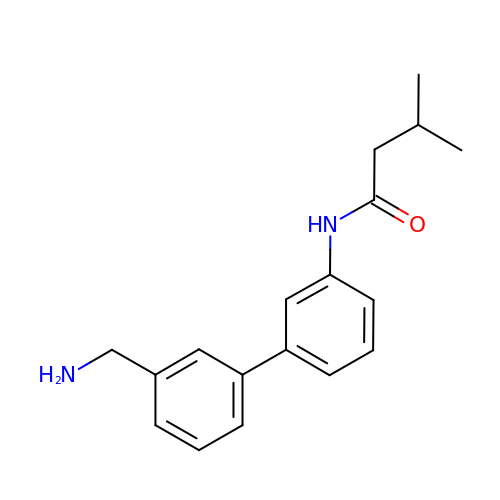~{N}-[3-[3-(aminomethyl)phenyl]phenyl]-3-methyl-butanamide | C18 H22 N2 O | ZTMBFIOZACRTLO-UHFFFAOYSA-N>[2x]MTTPPLLQLPVEVKKTELNGFWDTGAQITCIPEAFLKEEIPIGEAQIKTLHGTKLQSVYYLKFKVLGRKVEAEVTTSPFDYVIISPSDIPWYKPQPLELTVKLPVQDFKKELINKANINNEEKKQLAKLLDKYDVLWQQWENQVGHRKIPPHNIATGTVAPRPQRQYHINTKAKPSIQQVIDDLLKQGVLIKQTSVMNTPIYPVPKPDGKWRMVLDYRAVNKTVPLIGAQNQH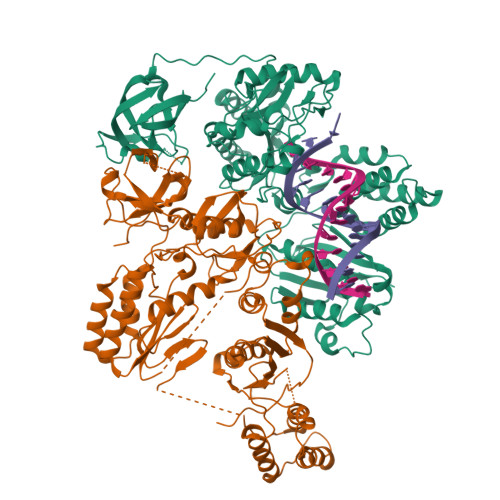SLGILTNLVRQKYKSTIDLSNGFWAHPITKDSQWITAFTWEGKQHVWTRLPQGFLNSPALFTADVVDLLKNIPGISVYVDDIYFSTETVSEHLKILEKVFKILLEAGYIVSLKKSALLRYEVTFLGFSITQTGRGLTSEFKDKIQNITSPRTLKELQSILGLFNFARNFVPNFSEIIKPLYSLISTAEGNNIKWTSEHTRYLEEIVSALNHAGNLEQRDNESPLVVKLNASPKTGYIRYYNKGGQKPIAYASHVFTNTELKFTPLEKLLVTMHKALIKAIDLALGQPIEVYSPIISMQKLQKTPLPERKALSTRWITWLSYLEDPRITFYYDKTLPDLKNVPETVTDKKPKMLPII>[2x]MSTVPELLARQVTRAPDAVAVVDRDRVLTYRELDELAGRLSGRLIGRGVRRGDRVAVLLDRSADLVVTLLAIWKAGAAYVPVDAGYPAPRVAFMVADSGASRMVCSAATRDGVPEGIEAIVVTDEEAFEASAAGA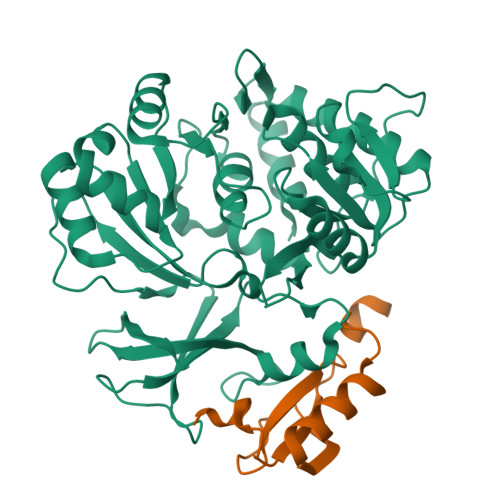RPGDLAYVMYTSGSTGIPKGVAVPHRSVAELAGNPGWAVEPGDAVLMHAPYAFDASLFEIWVPLVSGGRVVIAEPGPVDARRLREAISSGVTRAYLTAGSFRAVAEESPESFAGLREVLTGGDVVPAHAVARVRSACPRVRIRHLYGPTETTVCATWHLLEPGDEIGPVLPIGRPLPGRRAQVLDASLRAVAPGVIGDLYLSGAGLADGYLRRAGLTAERFVADPSAPGARMYRTGDLAQWTADGALLFAGRADDQGSHHHHHH;>[2x]MTNPFDNEDGSFLVLVNGEGQHSLWPAFAEVPDGWTGVHGPASRQDCLGYVEQNWTDLRPKSLISQISD> MERYENLFAQLNDRREGAFVPFVTLGDPGIEQSLKIIDTLIDAGADALELGVPFSDPLADGPTIQNANLRAFAAGVTPAQCFEMLAIIREKHPTIPIGLLMYANLVFNNGIDAFYARCEQVGVDSVLVADVPVEESAPFRQAALRHNIAPIFICPPNADDDLLRQVASYGRGYTYLLSRSGVVGAENRGALPLHHLIEKLKEYHAAPALQGFGISSPEQVSAAVRAGAAGAISGSAIVKIIEKNLASPKQMLAELRSFVSAMKAASRA;> TTLLNPYFGEFGGMYVPQILMPALNQLEEAFVSAQKDPEFQAQFADLLKNYAGRPTALTKCQNITAGTRTTLYLKREDLLHGGAHKTNQVLGQALLAKRMGK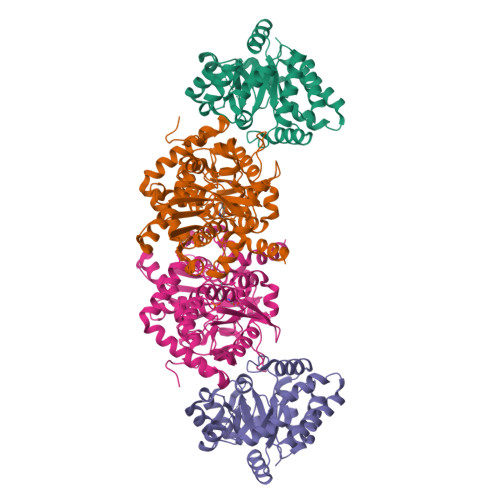SEIIAETGAGQHGVASALASALLGLKCRIYMGAKDVERQSPNVFRMRLMGAEVIPVHSGSATLKDACNEALRDWSGSYETAHYMLGTAAGPHPYPTIVREFQRMIGEETKAQILDKEGRLPDAVIACVGGGSNAIGMFADFINDTSVGLIGVEPGGHGIETGEHGAPLKHGRVGIYFGMKAPMMQTADGQIEESYSISAGLDFPSVGPQHAYLNSIGRADYVSITDDEALEAFKTLCRHEGIIPALESSHALAHALKMMREQPEKEQLLVVNLSGRGDKDIFTVHDILKARG> MLAKDKVALLIGNMNYREHPKLKAPLVDVYELTNLLRQLDFKVVSLLDLTEYEMRNAVDEFLLLLDKGVYGLLYYAGHGYENFGNSFMVPVDAPNPYRSENCLCVQNILKLMQEKETGLNVFLLDMCRKRNDYDDTIPILDALKVTANIVFGYATCQGAEAFEIQHSGLANGIFMKFLKDRLLEDKKI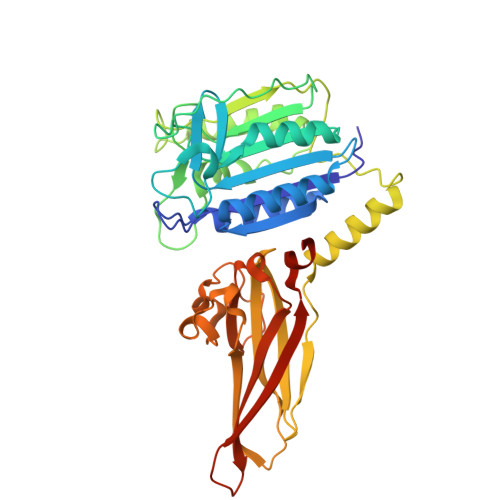TVLLDEVAEDMGKCHLTKGKQALEIRSSLSEKRALTDPIQGTEYSAESLVRNLQWAKAHELPESMCLKFDCGVQIQLGFAAEFSNVMIIYTSIVYKPPEIIMCDAYVTDFPLDLDIDPKDANKGTPEETGSYLVSKDLPKHCLYTRLSSLQKLKEHLVFTVCLSYQYSGLEDTVEDKQEVNVGKPLIAKLDMHRHHHHHH4-(furan-2-carbonyl)piperazine-1-carboxamide | C10 H13 N3 O3 | 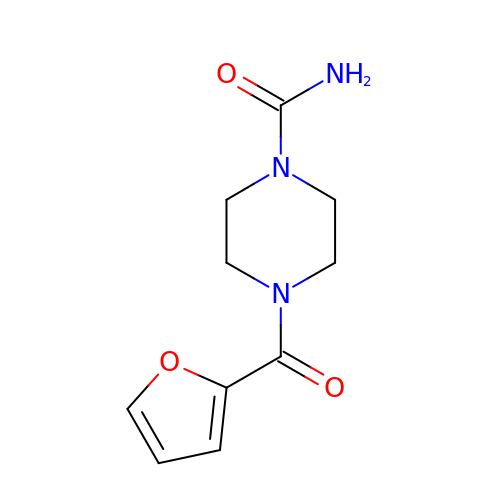TWRIXENNPDTMSQ-UHFFFAOYSA-N> MKINIRDSTMVRPATETPITNLWNSNVDLVIPRFHTPSVYFYRPTGASNFFDPQVMKEALSKALVPFYPMAGRLKRDDDGRIEIDCNGAGVLFVVADTPSVIDDFGDFAPTLNLRQLIPEVDH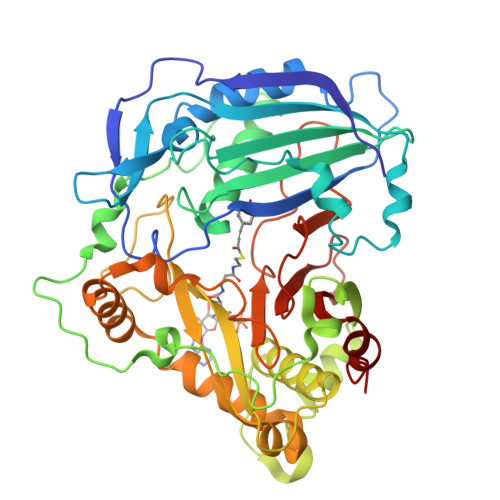SAGIHSFPLLVLQVTFFKCGGASLGVGMQHHAADGFSGLHFINTWSDMARGLDLTIPPFIDRTLLRARDPPQPAFHHVEYQPAPSMKIPLDPSKSGPENTTVSIFKLTRDQLVALKAKSKEDGNTVSYSSYEMLAGHVWRSVGKARGLPNDQETKLYIATDGRSRLRPQLPPGYFGNVIFTATPLAVAGDLLSKPTWYAAGQIHDFLVRMDDNYLRSALDYLEMQPDLSALVRGAHTYKCPNLGITSWVRLPIYDADFGWGRPIFMGPGGIPYEGLSFVLPSPTNDGSLSVAIALQSEHMKLFEKFLFEI>[2x]ADTIVAVELDTYPNTDIGDPSYPHIGIDIKSVRSKKTAKWNMQ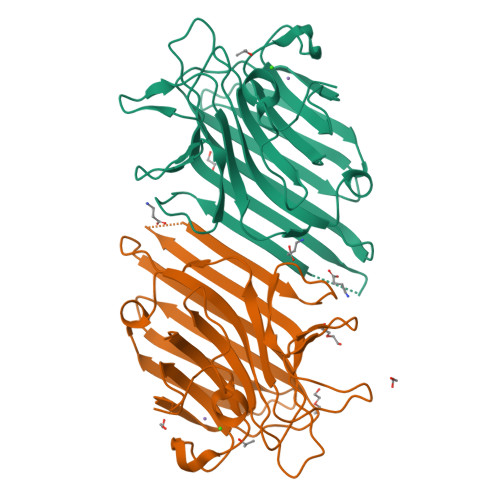NGKVGTAHIIYNSVGKRLSAVVSYPNGDSATVSYDVDLDNVLPEWVRVGLSASTGLYKETNTILSWSFTSKLKSNSTHETNALHFMFNQFSKDQKDLILQGDATTGTEGNLRLTRVSSNGSPQGSSVGRALFYAPVHIWESSAVVASFEATFTFLIKSPDSHPADGIAFFISNIDSSIPSGSTGRLLGLFPDAN>MSREEEQQRHNPYYFHSQGLRSRHESGEGEVKYLERFTERTELLRGIENYRVVILEANPNTFVLPYHKDAESVIVVTRGRATLTFVSQERRESFNLEYGDVIRVPAGATEYVINQDSNERLEMVKLLQPVNNPGQFREYYAAGAQSTESYLRVFSNDILVAALNTPRDRLERFFDQQEQREGVIIRASQEKLRALSQHAMSAGQRPWGRRSSGGPISLKSQRSSYSNQFGQFFEACPEEHRQLQEMDVLVNYAEIKRGAMMVPHYNSKATVVVYVVEGTGRFEMACPHDVSSQSYEYKGRREQEEEESSTGQFQKVTARLARGDIFVIPAGHPIAITASQNENLRLVGFGINGKNNQRNFLAGQNNIINQLEREAKELSFN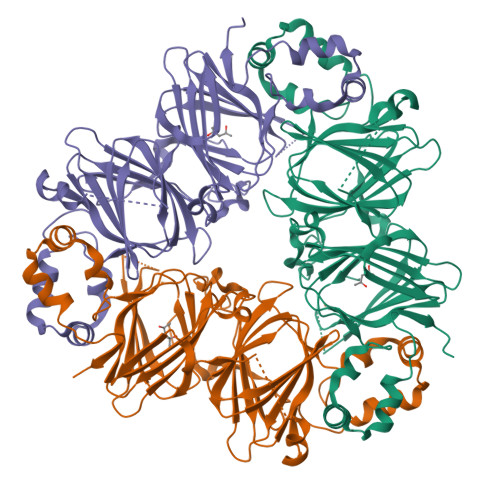MPREEIEEIFERQVESYFVPMERQSRRGQGRDHPLASILDFAGFF[6x]> MSVLSLIGELLVLFGTVFYLLSTLGLIRMPDVYNRMQTATKSATLGSLGVIIGTGIWALGEGFSVAWLTKAIVIA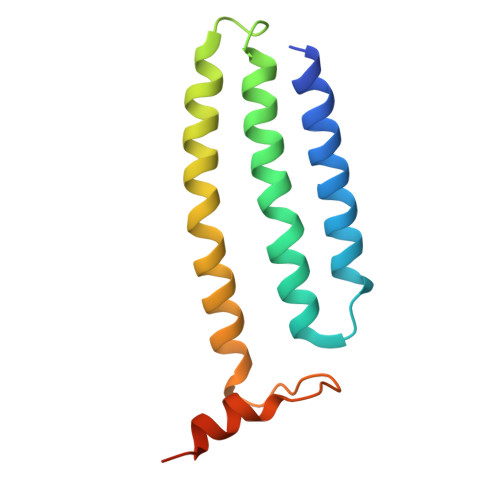AFLLLTNPISAHALIRAAYKSGIPLWEGSVVDKYKEHLERKKKEEGEQE> GPLGSSKVSEQLKCCSGILKEMFAKKHAAYAWPFYKPVDVEALGLHDYCDIIKHPMDM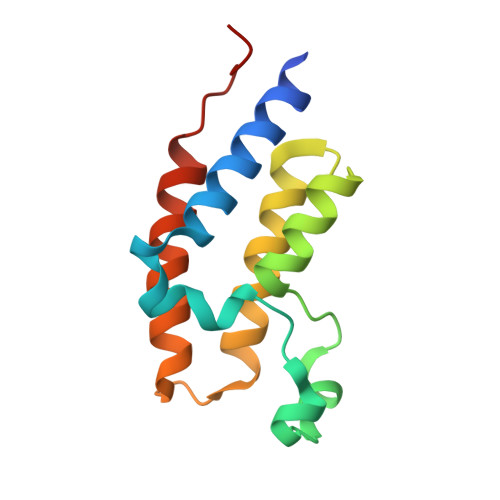STIKSKLEAREYRDAQEFGADVRLMFSNCYKYNPPDHEVVAMARKLQDVFEMRFAKMPDEPEEP~{N}-(3-chlorophenyl)-2-[(3,5-dimethyl-1,2-oxazol-4-yl)methoxy]benzamide 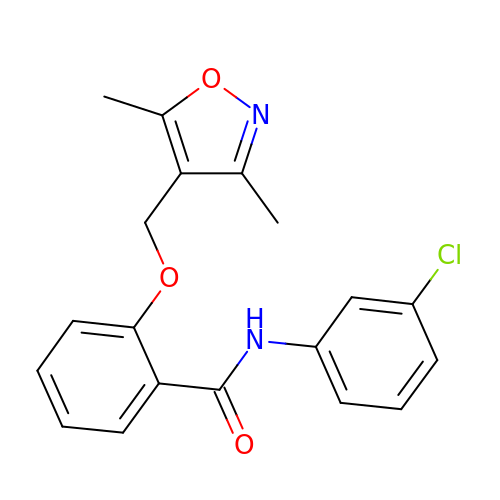| C19 H17 Cl N2 O3 | GBCRFZDGOAATHA-UHFFFAOYSA-N>MSWAETYKVNSDLQGEPLNFLSYLQDIKLNGLDSYVLFIGNARIWEELYLNSLYLFSDRGIRETVYTAFSETDIDNLFNKSTKLGEQLNAFYRTDIFSLGNADNVVKEMTIEHYNSLEEKFKAGYDRYVTREQEKSTIGAWFNSTFSLDNTDLENLTTIEEILANVEATNAILNNSNAIVALTMCKSSMDAVVASSNAMDLLGQYILRVTTESPVIRAI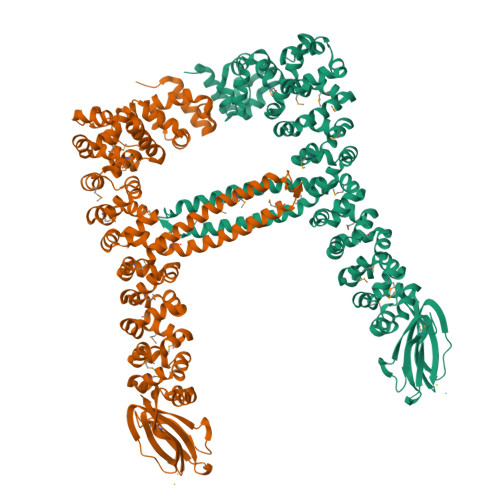LKNNVIRDAIINSDEAMTQISSNENSVMEIFNDLEATKVLVQNQNSINKILTNNVTVEKIIPNLLEMKYNLQTSLNYINTIKSNIASGKGQIMAITYNEEIFPILKNAVKNYDGMETTRNISQRDIEEKIKISDAILESSIAMATFANNSIIVNKVGDRVGIIESIFSKTVSLNAFMKSTTAINILVNKTTAFTKIANNSTAFNAMLTISENNVTIANNTTAMGIIANNAQAMSTVANNDTSISVFVNNTTAMGIIANSSTAMTKITLTGLALNRMVKSNTAKSILISKNSTLQTYKNNIQNTIQGSTAYFRTITGFADADDNPPQTINSTYVGITYCYGYKGNSYYGIVYHGYNTSIEAGRGNGYKDETKKFITLGGARYDQSGDGYFTYAMYQAI[4x]> MAKKTSSKGKLPPGPRPLPLLGNLLQMDRRGLLKSFLRFREKYGDVFTVHLGPRPVVMLCGVEAIREALVDKAEAFSGRGKIAMVDPFFRGYGVIFANGNRWKVLRRFSVTTMRDFGMGKRSVEERIQEEAQCLIEELRKSKGALMDPTFLFQSITANIICSIVFGKRFHYQDQEFLKMLNLFYQTFSLISSVFGQLFELFSGFLKHFPGAHRQVYKNLQEINAYIGHSVEKHRETLDPSAPRDLIDTYLLHMEKEKSNAHSEFSHQNLNLNTLSLFFAGTETTSTTLRYGFLL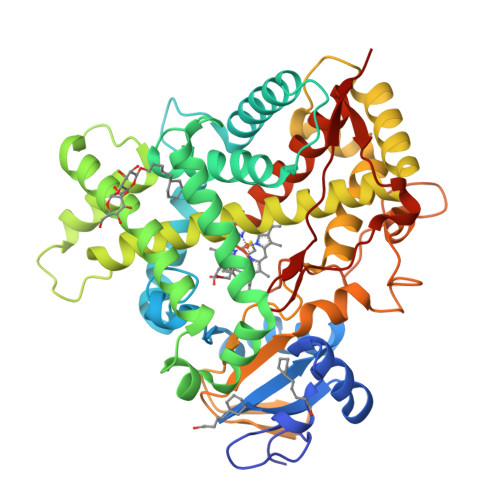MLKYPHVAERVYREIEQVIGPHRPPELHDRAKMPYTEAVIYEIQRFSDLLPMGVPHIVTQHTSFRGYIIPKDTEVFLILSTALHDPHYFEKPDAFNPDHFLDANGALKKTEAFIPFSLGKRICLGEGIARAELFLFFTTILQNFSMASPVAPEDIDLTPQECGVGKIPPTYQIRFLPRHHHH Complex I couples the transfer of two electrons from NADH to ubiquinone (Q) with the translocation of four protons across the membrane. The L-shaped complex is structured into a peripheral arm that protrudes into the aqueous milieu and catalyzes electron transfer with one FMN and 8–10 iron–sulfur ([Fe–S]) clusters, and a membrane arm embedded in the lipid bilayer that mediates proton translocation. We have determined structures of the electron-input module of complex I from the hyperthermophilic bacterium Aquifex aeolicus, encompassing subunits NuoE and NuoF that contain the FMN cofactor, the [4Fe–4S] cluster N3, and the [2Fe–2S] cluster N1a, respectively, both in the air-oxidized and dithionite-reduced states at resolutions up to 1.8 Å. Here, we show that the redox state of N1a regulates NADH oxidation in complex I by inducing a conformational change close to the NADH-binding site.

Crystals of A. aeolicus NuoEF contain two NuoEF heterodimers per asymmetric unit. Both monomers align with a root-mean-squared deviation (RMSD) of 0.17 Å for all atoms and will consequently not be discussed separately. NuoE and NuoF are very similar in structure to their homologues in T. thermophilus, Nqo1, and Nqo2, with a RMSD of 0.93 Å for 334 Cα atoms, in accordance with their high-sequence identity. However, our model of NuoEF contains 985 water molecules that are not detectable in the structure of the T. thermophilus complex I due to its lower resolution. However, the detailed analysis revealed that a single peptide bond, between E95F and S96F, undergoes a reversible flip, such that its carbonyl group points toward the flavin in the oxidized state, while it faces the loop coordinating N1a in the reduced state. This peptide bond is located in the active site of the enzyme between the FMN cofactor and cluster N1a. In addition, two conserved water molecules are present in the active site in the oxidized state of NuoEF. The disulfide bond between C144 and C172 found in T. thermophilus complex I24 is not present in the A. aeolicus ortholog.

>[2x]MFKTEFEFPEELKTKLQEHINYFPKKRQAILLCLHEIQNYYGYIPPESLKPLADMLELPLNHVEGVVAFYDMFDREDKAKYRIRVCVSIVCHLMGTNKLLKALENILGIKPGEVTPDGKFKIVPVQCLGACSEAPVFMVNDDEYKFESEVQLNEILSRYT;>MRSYPAIPRIYAETTLNMLLKRAKKPRVHSIDEYLKDGGYQALEKALNMSPEEIIDWVDKSTLRGRGGAGFPTGKKWKFAVQNPGPRYFICNADESEPGTFKDRIIIERDPHLLIEGIIISSYAIGANEAYIYIRGEYPAGYYILRDAIEEAKKKGFLGKNILGSGFDLEIYVARGAGAYICGEETALIESLEGKRGHPRLKPPYPVQKGLWGKPTVVNNVETIANVPFIISMGWEEYRYIGPSDYAGPKLFPVSGKVKKPGVYELPMNTTLREVIFKYAGGTLGNKKVKAVFSGALDCFSSEELDIPMDYSPLGFGGTGTVIVLTEEDDIVEAALKIAEFYEHETCGQCTPCRVGCYEQANLLEKIYKGEATEQDWEGFDFVNRNIQPTSICGLGAVAGRLIRQTLEKFPEEWEKYRKKSASLPLAGHHHHHH[2x]>[2x]RSPVFTDNSSPPAVPQSFQVAHLHAPTGSGKSTKVPAAYAAQGYKVLVLNPS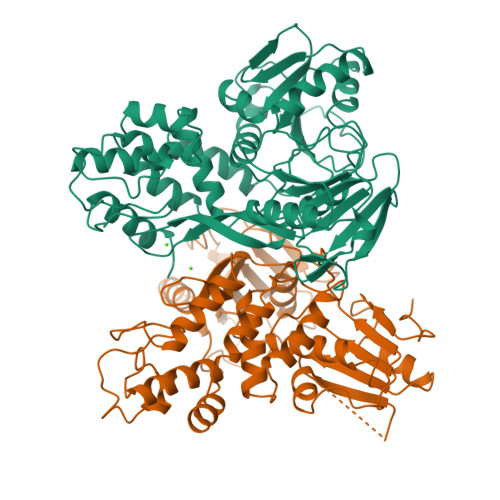VAATLGFGAYMSKAHGVDPNIRTGVRTITTGSPITYSTYGKFLADGGCSGGAYDIIICDECHSTDATSILGIGTVLDQAETAGARLVVLATATPPGSVTVSHPNIEEVALSTTGEIPFYGKAIPLEVIKGGRHLIFCHSKKKCDELAAKLVALGINAVAYYRGLDVSVIPTNGDVVVVSTDALMTGFTGDFDSVIDCNTCVTQTVDFSLDPTFTIETTTLPQDAVSRTQRRGRTGRGKPGIYRFVAPGERPSGMFDSSVLCECYDAGCAWYELMPAETTVRLRAYMNTPGLPVCQDHLEFWEGVFTGLTHIDAHFLSQTKQSGENFPYLVAYQATVCARAQAPPPSWDQMWKCLIRLKPTLHGPTPLLYRLGAVQNEVTLTHPITKYIMTCMSADLEVV> EPKKYAVTDDYQLSKQVLGLGVNGKVLECFHRRTGQKCALKLLYDSPKARQEVDHHWQASGGPHIVCILDVYENMHHGKRCLLIIMECMEGGELFSRIQERGDQAFTEREAAEIMRDIGT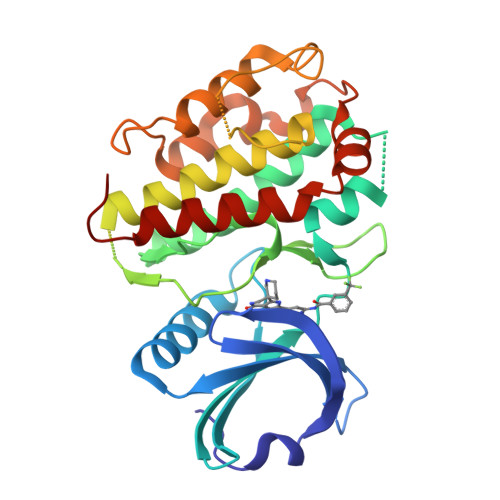AIQFLHSHNIAHRDVKPENLLYTSKEKDAVLKLTDFGFAKETTQNALQTPCYTPYYVAPEVLGPEKYDKSCDMWSLGVIMYILLCGFPPFYSNTGQAISPGMKRRIRLGQYGFPNPEWSEVSEDAKQLIRLLLKTDPTERLTITQFMNHPWINQSMVVPQTPLHTARVLQEDKDHWDEVKEEMTSALATMRVDYDQV> GMTEDSQRNFRSVYYEKVGFRGVEEKKSLEILLKDDRLDTEKLCTFSQRFPLPSMYRALVWKVLLGILPPHHESHAKVMMYRKEQYLDVLHALKVVRFVSDATPQAEVYLRMYQLESGKLPRSPSFPLEPDDEVFLAIAKAMEEMVEDSVDCYWITRRFVNQLNTKYRDSLPQLPKAFEQYLNLEDGRLLTHLRMCSAAPKLPYDLWFKRCFAGCLPESSLQRVWDKVVSGSCKILVFVAVEILLTFKIKVMALNSAEKITKFLENIPQDSSDAIVS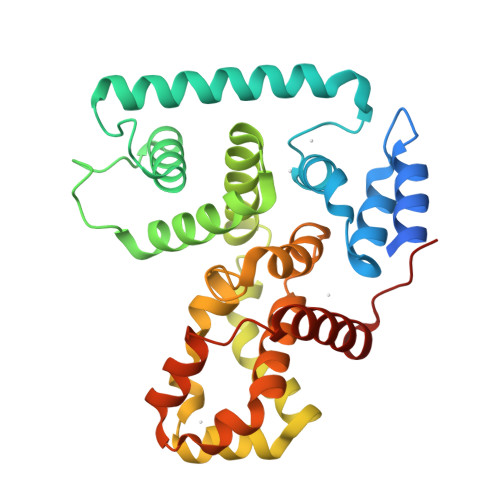KAIDLWHKHCGTPVHSS4-fluorobenzoic acid | C7 H5 F O2 | 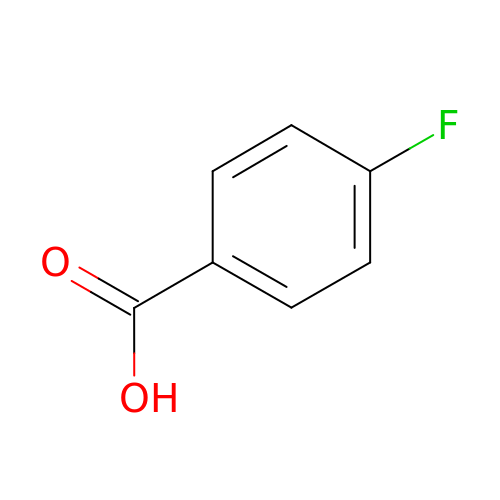BBYDXOIZLAWGSL-UHFFFAOYSA-N>KVDLQSLPTRAYLDQTVVPILLQGMAVLAKERPPNPIEFLASY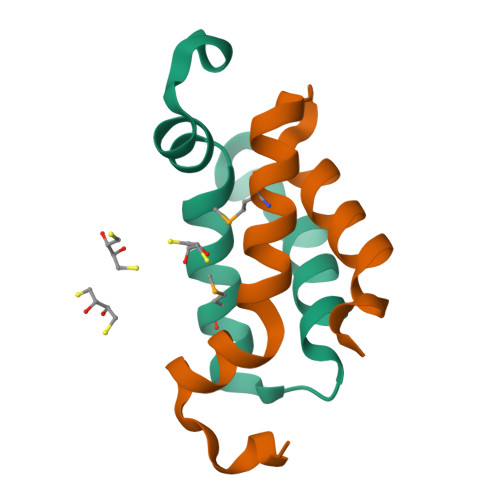LLKNKAQFEDRN[4x]>MYELTPEQRTLQTQARELAQSVFASTAVQTDLTEQYPWDNVAQLRDAGFMGMMLPTSVGGRGLSTLDTVIVIEEMAKACATMGRITVDSNLGAIGAITKYGSEEQIKLAADLVLAGDKPAICISEPNAGSAASEMTTRADKNGDHYILNGEKYWITGGGVSKLHLIFARVFDDGVEQGIGAFITVLDDHGPEGLKVGRRLYAMGVRGIPETHLEFHDLKIHKSMMITFPDGLKRGFAALMSAYNAQRVGAGAVALGIAQCAFEEGVAY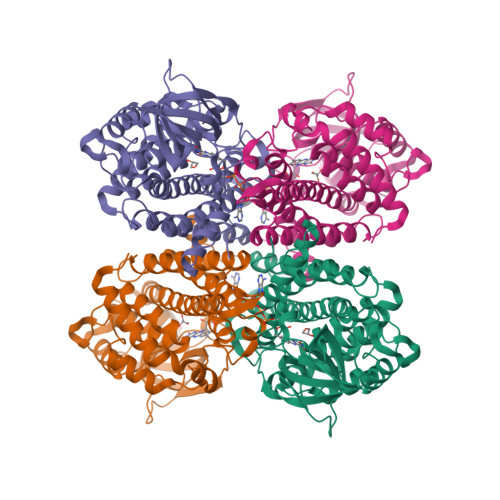LKRREQFGRPLAEFQGLQWMVADMSVQLEAARLMLRSAAVSGETFPDINKAAQAKIFAAETANKVTNDALQFFGSSGYGRHNPMERHVRDARMFTIAGGTAQILRTQVASKILDMKLPQTRDGYLKAAQNSKR[2x]> MPHPRRYHSSERGSRGSYREHYRSRKHKRRRSRSWSSSSDRTRRRRREDSYHVRSRSSYDDRSSDRRVYDRRYCGSYRRNDYSRDRGDAYYDTDYRHSYEYQRENSSYRSQRSSRRKHRRRRRRSRTFSRSSSQHSSRRAKSVEDDAEGHLIYHVGDWLQERYEIVSTLGEGTFGRVVQCVDHRRGGARVALKIIKNVEKYKEAARLEINVLEKINEKDPDNKNLCVQMFDWFDYHGHMCISFELLGLSTFDFLKDNNYLPYPIHQVRHMAFQLCQAVKFLHDNKLTHTDLKPENILFVNSDYELTYNLEKKRDERSVKSTAVRVVDFGSATFDHEHHSTIVSTRHYRAPEVILELGWSQPCDVWSIGCIIFEYYVGFTLFQTHDNREHLAMMERILGPIPSRMIRKTRKQKYFYRGRLDWDENTSAGRYVRENCKPLRRYLTSEAEEHHQLFDLIESMLEYEPAKRLTLGEALQHPFFARLRAEPPNKLWDSSRDISR

CLKs are dual-specificity kinases that are activated by autophosphorylating their own tyrosine residues and subsequently phosphorylate the serine/threonine residues of the SR protein. Later, CX-4945 was revealed to have a strong inhibitory activity on CLKs; IC50 values of 82.3 nM (CLK1), 3.8 nM (CLK2), and 90.0 nM (CLK3). In order to elucidate the selective inhibitory effect of CX-4945 on CLKs, we determined the structures of CLK1, CLK2, and CLK3 in complex with CX-4945. The overall structure of the CLK catalytic domain contained 12 β-strands and 10 α-helices that could be divided into the N-lobe and C-lobe, which are typical forms of the kinase.

Out of CLKs, CLK2 was most strongly inhibited by CX-4945 with 3.8 nM of IC50 in vitro, which is quite noteworthy in that most of CLK inhibitors are more potent on CLK1/CLK4 than CLK2. Moreover, its inhibitory potency on CLK2 was similar to or even higher than that on CK2 (14.7 nM of IC50). CLK2 had the longest N-terminus with an extra eight residues; in contrast, CLK1 had the shortest N-terminus. For the β-hairpin insertion structure, CLK2 had a complete conformation, whereas CLK1 showed a partially disordered loop. The interactions between CX-4945 and CLK2 were highly similar except for the carboxyl group of CX-4945. The carboxyl group also directly interacted with Lys193, and water-mediated interactions were observed only with Glu208 and not Asp327 because there was no water molecule between them. Intriguingly, the charge distribution pattern of CLK2 was the weakest compared with that of CLK1 and CLK3, indicating its preference to bind to the hydrophobic benzonaphthyridine ring of CX-4945. Therefore, based on the size and electrostatic charge distribution of the active site, the binding of CLK2 to CX-4945 could be stronger than the binding of the other two CLKs. Third, out of three CLKs, CLK2 has the weakest charge distribution, favoring its hydrophobic interactions with benzonaphthyridine ring. Together, these results support the relatively favorable binding of CX-4945 with CLK2 over CLK1 and CLK3, which is consistent with its stronger effect on CLK2 that were defined in the previous study.> MDQETIDTDYDVIV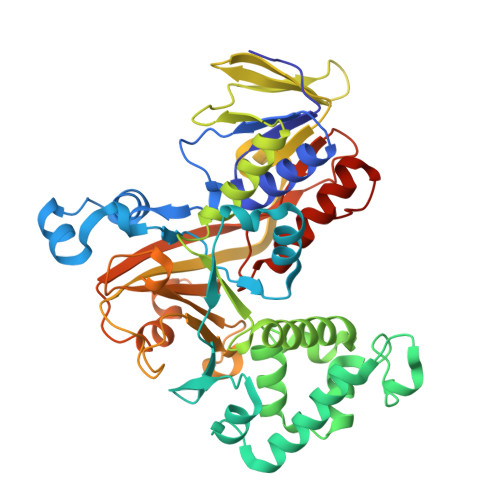LGTGITECILSGLLSVDGKKVLHIDKQDHYGGEAASVTLSQLYEKFKQNPISKEERESKFGKDRDWNVDLIPKFLMANGELTNILIHTDVTRYVDFKQVSGSYVFKQGKIYKVPANEIEAISSPLMGIFEKRRMKKFLEWISSYKEDDLSTHQGLDLDKNTMDEVYYKFGLGNSTKEFIGHAMALWTNDDYLQQPARPSFERILLYCQSVARYGKSPYLYPMYGLGELPQGFARLSAIYGGTYMLDTPIDEVLYKKDTGKFEGVKTKLGTFKAPLVIADPTYFPEKCKSTGQRVIRAICILNHPVPNTSNADSLQIIIPQSQLGRKSDIYVAIVSDAHNVCSKGHYLAIISTIIETDKPHIELEPAFKLLGPIEEKFMGIAELFEPREDGSKDNIYLSRSYDASSHFESMTDDVKDIYFRVTGHPLVLKQRQEQEKQ N-({[(1R,3S)-3-(6-amino-9H-purin-9-yl)cyclopentyl]methyl}sulfamoyl)-5-[(3aS,4S,6aR)-2-oxohexahydro-1H-thieno[3,4-d]imidazol-4-yl]pentanamide 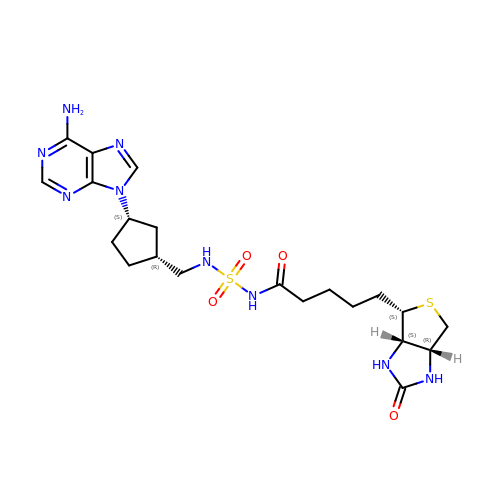| C21 H31 N9 O4 S2 | WZGWWAMUOOWNHU-MDLJMBGESA-N> SDRAEVRNIPFKLGMSLTVGGVVNSNATRFSINVGESTDSIAMHMDHRFSYGADQNVLVLNSLVHNVGWQQEERSKKFPFTKGDHFQITITFDTHTFYIQLSNGETVEFPNRNKDAAF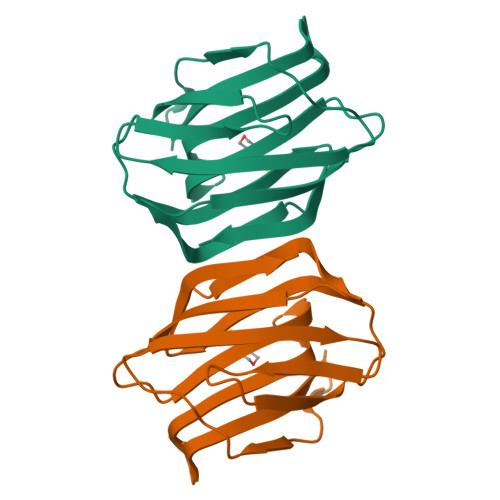NLIYLAGDARLTFVRLE>[6x]GANAMAHMGKTLRFEIVSGVNKGYFHTNSQSESLDLVGGIWQKIAKEEFEKSNIYVSAVIKPSKTVYNQEWGCPENGEETVVLTGVANEEFVDDIEKWKDTVIKLAKELKNQMKQSTLTCEF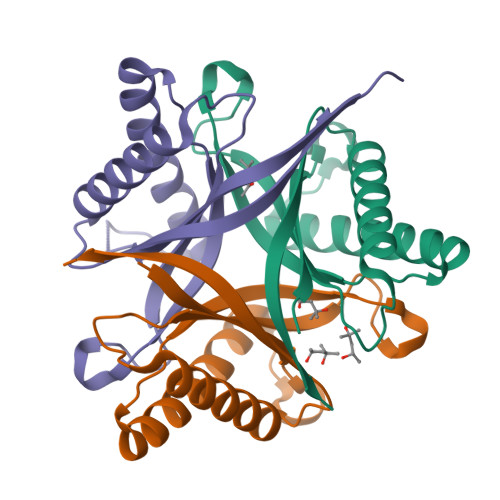IETELHYFK3-[5-[5-(4-METHYL-PIPERAZIN-1-YL)-1H-IMIDAZO[4,5-B]PYRIDIN-2-YL]-BENZIMIDAZOL-2-YL]-PHENOL 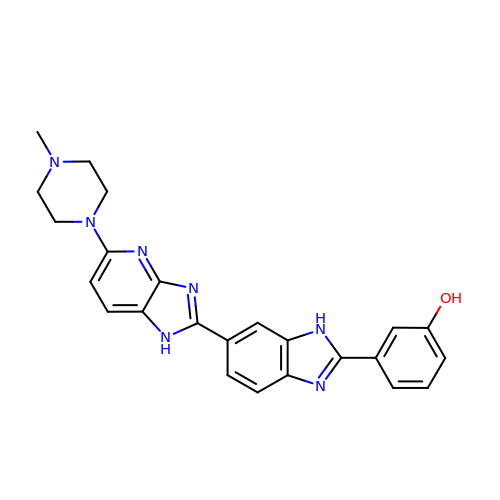| C24 H23 N7 O | VDFACTPXXYZXTP-UHFFFAOYSA-N> MGNTATEFDGPYVITPISGQSTAYWICDNRLKTTSIEKLQVNRPEHCGDLPETKLSSEIKQIMPDTYLGIKKVVALSDVHGQYDVLLTLLKKQKIIDSDGNWAFGEGHMVMTGDMFDRGHQVNEVLWFMYQLDQQARDAGGMVHLLMGNHEQMVLGGDLRYVHQRYDIATTLINRPYNKLYGADTEIGQWLRSKNTIIKINDVLYMHGGISSEWISRELTLDKANALYRANVDASKKSLKADDLLNFLFFGNGPTWYRGYFSETFTEAELDTILQHFNVNHIVVGHTSQE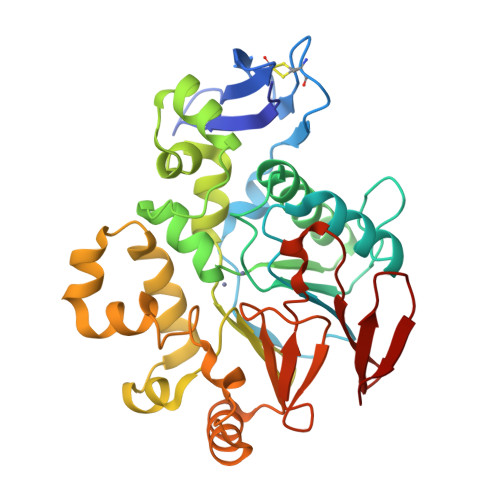RVLGLFHNKVIAVDSSIKVGKSGELLLLENNRLIRGLYDGTRETLQ>RLGEVEARQVATPREAQQLAQRQEAPKGEGLLSRLGAALARPFVAIIEWLGKLLGSR[2x];>MNPLYRAAIHQLFLALDLPTPNDEESVLSLQVGPHLCHLAEHPTDHLLMFTRLEGQGDATANEQNLFS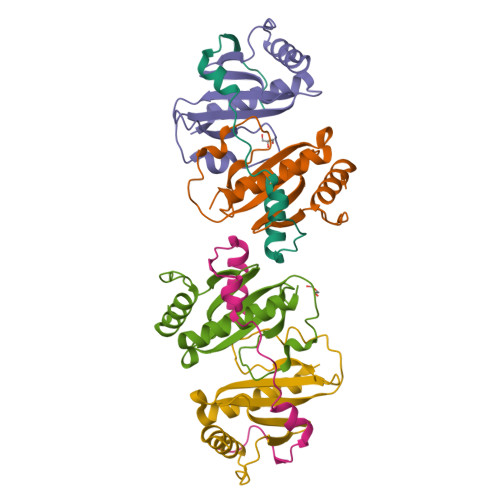QDPCKPILGRDPESGERLLWNRQPLQLLDRAQIHHQLEQLVAAAEELR[4x]>[2x]MEKRMSTQQRAAGNACPTAAFSFDPARLAQRRRWAGAFAALCGLALSPSALLAEEHSQHQDHAVELAPSVVTGVAQSSPLTIVTNPKEPRQPVPASDGADYLKTIPGFAVIRNGGSNGDPVLRGMFGSRLNILTNGGMMLGACPNRMDAPTSYISPETYDKLTVIKGPQTVLWGPGASAGTILFEREPERFGELGSRVNASLLAGSNGRFDKVLDAAAGNRLGYLRFTGNHAQSDDYEDGAGNTVPSRWKKWNGDVAVGWTPDEDTLIELTAGKGDGEARYAGRGMDGSQFKRESLGLRFVKS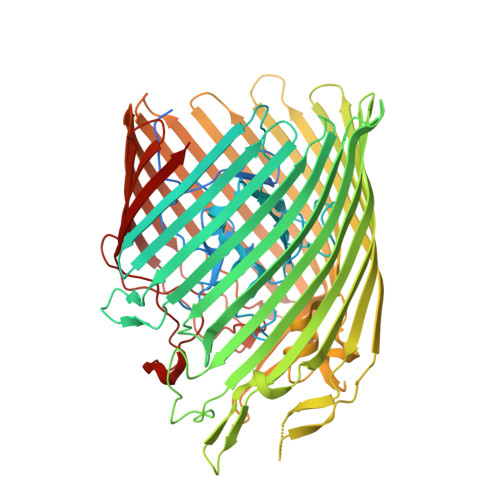NVSDVLEKVEAQVYYNYADHIHDNFRLRTPDPSSMMPMPMASQVDRRTLGGRLAATWRWDDFKLVTGVDAMRNEHRARGSKYDMMTDYYTDADQFPWSKDAVFHNYGAFGELTWFAAERDRLIGGLRLDRASVKDYRQTLKSGHMGHAMANPTANDTRADTLPSGFVRYEHDLADSPTTLYAGLGHAERFPDYWELFSPKRGPNGSVNAFDKIKPEKTTQLDFGLQYNGDKLQAWASGYVGVVQDFILFSYREGMMGSSTQATNVDARIMGGELGASYQLTGNWKTDASLAYAWGKNSSDDRALPQIPPLEARFGLTYEEGDWSAGSLWRVVAPQNRIARDQGNVVGKDFDKSAGFGVFSLNGAYRVTRNVKLSAGVDNLFDKDYTEHLNKAGDAGFGFSANETVPEPGRTFWTKVDFSF>AVTCGQVDANLAPCVPFLTQGGEPGAACCSGVKTLNGNAQSPDDRKTACNCIKAAANRYPNLKDDAAQSLPSKCGI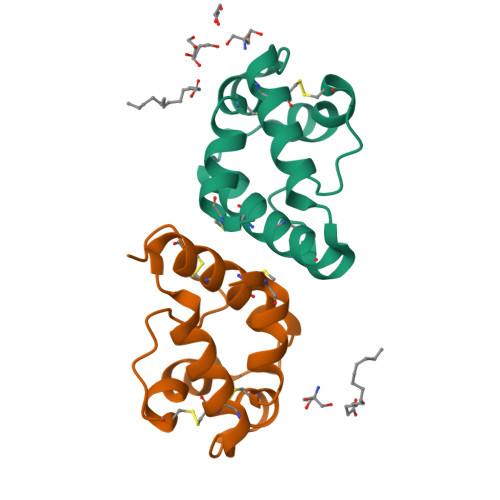SLNVPISRTINCDTIS[2x]>MRDPLDFQSIIMKLQQFWAEQGSLIWQPYYTQVGAGTMNPATFLRVLGPEPWNVAYVEPSIRPDDGRYGENPNRLQQHYQFQVILKPDPGNPQEIYLRSLEALGIDPREHDIRFVEDNWESPALGAWGLGWEVWLDGLEITQFTYFQQAGGMVLEPVSVEITYGLERIAMALQRVSNFRDIRWNAERTYGDVNLQGEREHSTYYFEVADVERLRQMFALFEAEAEAALARGLVLPAHDYVLKSSHTFNVLDTRGAVGVTERQVLFARMRDMARRVAEAYVAQRQALGFPWLKPTAQVSEAPAVREAPRSIPEQETLLIEIGTEELPPADLEAALAQLRQRVPALLDELHLPHGDVQVWGTPRRLVVWVEDLAGRQPDRELIIKGPPANRAFDAEGRPTAAAEGFARSKGVPVEALTVAEMDGGRYVVAHVRETGRPAVEVLAEVLPGVIADLRFERSMRWNSSGVAFSRPIRWLVALHGETVIPFTYAGLTSGRVTRGLRFAEPATFALSHPRDYRIFLERQGVVVEPEIRRARIAEQARTLIADVGGDPEHLDEAVLNEVTHLVEAPTALRGRFEDEYLRLPEEVLVSVM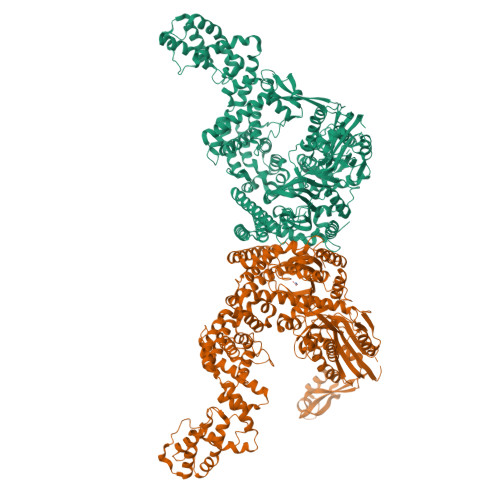KKHQRYFPVYTREGQLLPYFIAVRNGGKEGLDVVTDGNEQVIRARFADAAYFIREDLKHPLEYYLPRLSTLTFQAKLGSMLDKTHRIEVLVERLIPMVGLEAEDAAAVRRAAHLSKADLVTHMVVEMTSLQGVMGRYYALQSGEPRAVAEAIFEAYLPRFAGDRYPETPAGLVLGLADRLDTLMGLFAVGLAPTGTKDPFALRRAALGLVQNLIHWNLDFDLRQGLEAAAQGLPVPVSPEAKMESLEFIVGRLQNELLEQGYRYDVVAAVLAAQGHNPAATARGVRELSAWVSRSDWNTILPAYARSVRITRDQTERFAIDPARLVEPAEKHLLSALLQAEVTPRRPGSVEDFFQVFLPMIPVINRFFDEVLVMAEDAGLRANRLGLLQRIVALADGVADFSKLEGFENLYFQGHHHHHH[2x]Bacteriophage Exclusion (BREX) systems recognise and methylate 6 bp non-palindromic motifs within the host genome, and prevent replication of non-methylated phage DNA that encodes these same motifs. The PglX N-terminal domain encodes the methyltransferase, whereas the C-terminal domain is for motif recognition. Our data demonstrate that PglX is used to recognise specific DNA sequences for BREX activity, contributing to motif recognition for both phage defence and host methylation. As a result, the PglX structure, and lack of nuclease motifs and potential aligned catalytic residues, supports PglX acting as a methyltransferase only, and not acting as a restriction enzyme.

Ocr is the T7-encoded restriction system inhibitor that blocks phage defence activity of the E. coli BREX system. Within the asymmetric unit, PglX-SAM binds to a protomer of Ocr as a 1:1 complex, with the single protomer of Ocr binding along the positively charged region of the C-terminal domain of PglX. In this complex, the Ocr protomers perfectly align and abut one another, forming the equivalent of a solution state dimer, and the size matches our analytical SEC. We therefore concluded that this heterotetrameric form represented the solution state of the PglX-SAM:Ocr complex. Six salt bridges are produced between R79, D35, D42, D62, D76 and E109 of Ocr and D1213, K1201, K1097, K1070, K1110, and K516 of PglX, respectively. The complex is stabilised by a number of hydrogen bonds between Ocr and the C-terminal domain of PglX. Also visible in the PglX-SAM:Ocr structure is a bound SAM molecule, in the same ligand binding position as seen in the PglX-SAM structure. The PglX molecules from the PglX-SAM and PglX-SAM:Ocr structures align closely with an RMSD of 1.34 Å (9564 atoms), suggesting that binding of Ocr does not elicit any substantive domain movement. Within PglX, there were again two regions of the sequence which could not be modelled due to insufficient density (residues 54–55 and 413–420). Collectively, these data suggest that Ocr acts as a DNA mimic, capable of sequestering PglX and therefore blocking BREX activity by preventing recognition of target DNA.

> MNTNNIKKYAPQARNQFRDAVIQKLTTLGISADKKGNLQIADAELVGETMRYGQFDYPKSTLTRRDRLVKRAREQGFDVLVEHCAYTWFNRLCAIRYMEIHGYLDHGFHMLSHPDNPTGFEVLDHVPEVAEALLPEKKAQLVEMKLSGNQDEAIYRELLLAQCHALHRAMPFLFEAVDDEAELLLPDNLTRTDSILRGLVDGIPEEDWQEVEVIGWLYQFYISEKKDAVIGKVVKSEDIPAATQLFTPNWIVQYLVQNSVGRQWLQTYPDSPLKGKMDYYIEPAEQTPEVQAQLAAITPASIEPESIKVLDPACGSGHILIEVYNVLKNIYEERGYRARDIPQLILENNIFGLDIDDRAAQLSGFALLMMARQDDRRIFTRDVRLNIVSLQESLHLDIAKLWQQLNFHQQNQTGSMGDMFAENTALAHTDSAEYQLLMRTLKRFVNAKTLGSLIQVPQEEEAELKAFLEALYRMEQEGDFQQKAAAKAFIPYIQQAWILAQRYDAVVANPPYMGGKGMNSELKEFAKNNFPDSKADLFAMFMQNAFSLLKENGFNAQVNMQSWMFLSSYEALRNWLLDNKTFITMAHLGARAFGQISGEVVQTTAWVIKNQHSERYQPVFFRLIDGREEVKKSDLLLRKNIFDKFTQHDFKNIPGMPIAYWIDLPSLLSFRHHKKLGEKIALKAGMSTGDNIKFQRYWYEVSIKKTLITNKESNTKIDIHNIKWFPCSSGGEYRKWYGNNEIVVNWENNGYEIRNFKFENGKTRSAVRNDEYYFREGITWSKISQGNFCVRYRPKGFVFDDTGRCGFSNNKNELLYAAGLMCTPVVNHYLSILAPTLSFTSGELASVPYPEIEDEIIELVTNAIEIAKNDWDSQEQSWDYVCSPLLEHNSTQLLRNIYKQKINTNIKLVETLLLIENTINNIFIDKLQLDKTIIKAVLQSEITLLCNPNYRYKNIQDHTDLTNKYYTDITIDILSYIIGCMMGRYSLDREGLVYAHEGNKGFAELVAEDAYKTFPADNDGILPLMDDEWFDDDVTSRVKEFVRTVWGEEHLQENLEFIAESLCLYAIKPKKGESALDTIRRYLSTQFWKDHMKMYKKRPIYWLFSSGKEKAFECLVYLHRYNDATLARMRTEYVVPLLARYQANIDRLNEQVDGASGGEATRLKRERDSLSKKFNELRSFDDRLRHYADMRISIDLDDGVKVNYGKFGDLLADVKAITGNAPEII;> MAMSNMTYNNVFDHAYEMLKENIRYDDIRDTDDLHDAIHMAADNAVPHYYADIFSVMASEGIDLEFEDSGLMPDTKDVIRILQARIYEQLTIDLWEDAEDLLNEYLEEVEEYEEDEE>AECSVDIQGNDQMQFNTNAITVDKSCKQFCVNLSHPGNL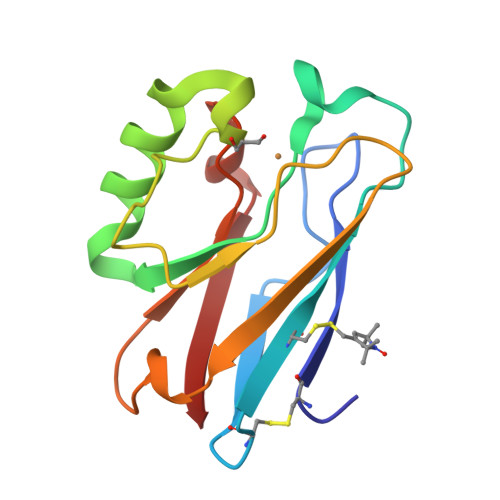PKNVMGHNWVLSTAADMQGVVTDGMASGLDKDYLKPDDSRVIAHTKLIGSGEKDSVTFDVSKLKEGEQYMFFCTFPGHSALMKGTLTLK[16x]(2E,4E)-3-methyl-5-(2,3,6,7-tetrahydro-1H,5H-pyrido[3,2,1-ij]quinolin-9-yl)penta-2,4-dienal | C18 H21 N O | 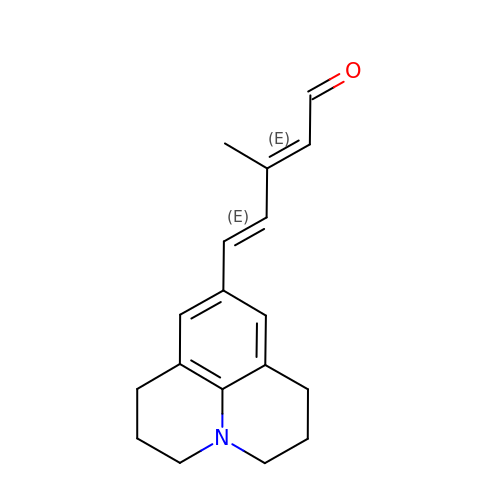LJFLJZQWTCHPOI-MDVYSFJGSA-N cis-4-methylcyclohexanamine | C7 H15 N | 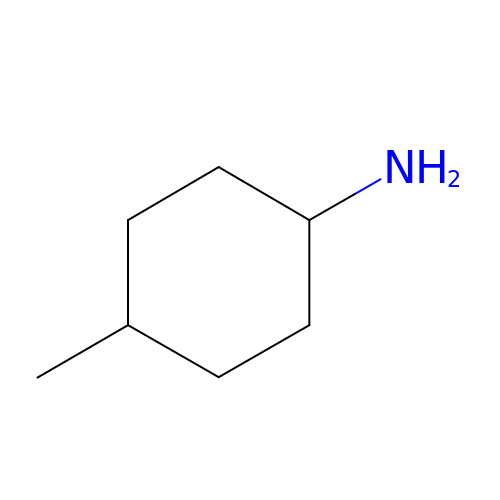KSMVBYPXNKCPAJ-KNVOCYPGSA-N(6S)-2-amino-6-(3'-methoxybiphenyl-3-yl)-3,6-dimethyl-5,6-dihydropyrimidin-4(3H)-one 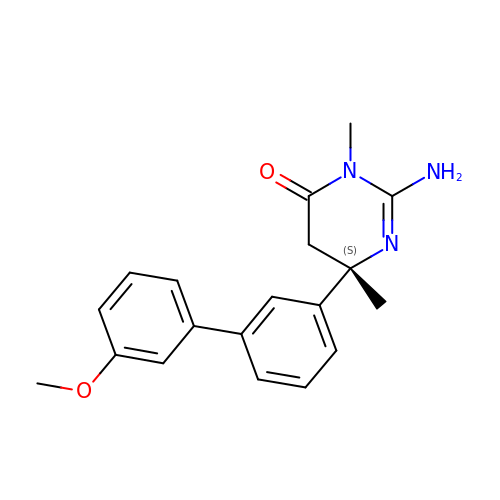| C19 H21 N3 O2 | LQOCXPOKEPYGTJ-IBGZPJMESA-N3-chloranyl-~{N}-(4,5-dihydro-1,3-thiazol-2-yl)-6-fluoranyl-1-benzothiophene-2-carboxamide | C12 H8 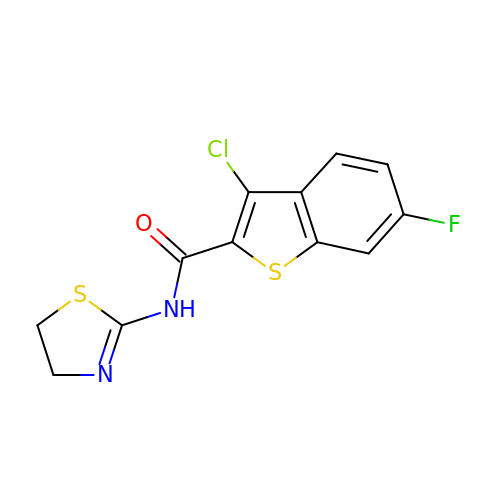Cl F N2 O S2 | WIYIHXHWMONCNB-UHFFFAOYSA-N> MSTSEQKDLTVSVPWSVQEDLLLDVAAPLLDESVELGETDSWFYLRENHGGRPFLRLRFASRSPSVERRLKSRILAHVGPTIDAGDVFTYQPYNHEHDWLGGTAGLGLAENFWTETTPLALDTLRATRGN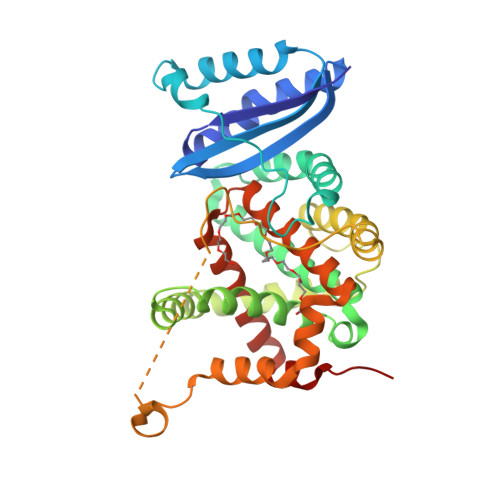RALRLAVAFDFLVCTGVMLAPHLPPSIAKFGYKAGYLSYLATFEGYMLLIRDPEGTRAKHAQRYEKNRELLRPRLRTLVEQMSEPDGELTDVPELAREWLVRLRDYVPALQKGFDEGRFYLYATPRKAETAKLTPSPDGLYRRPDVEWLSDLPEPPVAGIHRAIADNTYYQGMIREDRRFLASRLAQAYTNWHLYRLGFLLADRYTLFYLIARAFEEEYDLDAAALIRSVRPEAEVAG9-(3-azidopropyl)-8-bromanyl-purin-6-amine 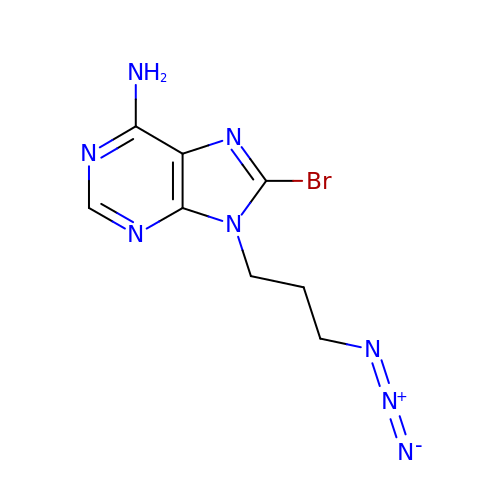| C8 H9 Br N8 | MCUGUHUWEQYYKC-UHFFFAOYSA-N> NPVENYIDSVLNEVLVVPNIQPSTS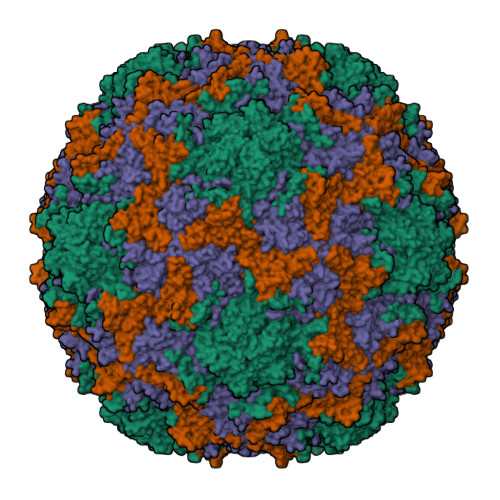VSSHAAPALDAAETGHTSSVQPEDMIETRYVITDQTRDETSIESFLGRSGCIAMIEFNTSSDKTEHDKIGKGFKTWKVSLQEMAQIRRKYELFTYTRFDSEITIVTAAAAQGNDSGHIVLQFMYVPPGAPVPEKRDDYTWQSGTNASVFWQEGQPYPRFTIPFMSIASAYYMFYDGYDGDSAASKYGSVVTNDMGTICVRIVTSNQKHDSNIVCRIYHKAKHIKAWCPRPPRAVAYQHTHSTNYIPSNGEATTQIKTRPDVFTVTNVGPSSMF;> SPTVEACGYSDRLIQITRGDSTITSQDTANAVVAYGVWPSYLTPDDATAIDKPTQPDTSSNRFYTLDSRSWTSASSGWWWKLPDALKNMGIFGENMFYHFLGRSGYTIHVQCNSSKFHQGLLIVAAIPEHQLASATSGNVSVGYNHTHPGEQGREVVPSRTSSDNKRPSDDSWLNFDGTLLGNLPIYPHQYINLRTNNSATLILPYVNAVPMDSMLRHNNWSLVIIPICPLQVQPGGTQSIPITVSISPMFSEFSGPRSKVVFSTTQ;> GLPVMLTPGSGQFLTTDDTQSPSAFPYFHPTKEIFIPGQVRNLIEMCQVDTLIPVNNTQENVRSVNMYTVDLRTQVDLAKEVFSIPVDIASQPLATTLIGELASYYTHWTGSLRFSFMFCGSASSTLKLLIAYTPPGVGKPKSRREAMLGTHLVWDVGLQSTASLVVPWVSASHFRFTTPDTYSSAGYITCWYQTNFVVPDSTPDNAKMVCMVSACKDFCLRLARDTNLHTQEGVLTQ;> MGAQVSRQNVGTHSTQNSVSNGSSLNYFNINYFKDAASSGASRLDFSQDPSKFTDPVKDVLEKGIPTLQ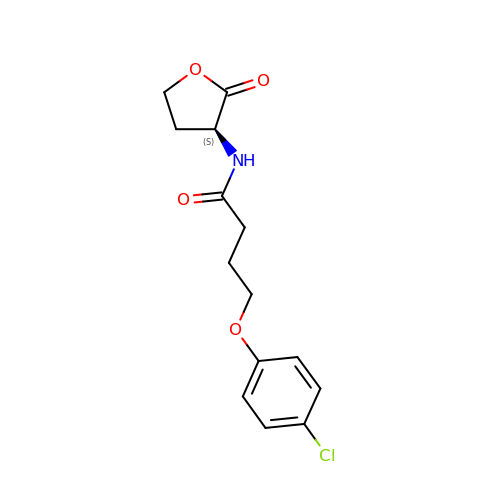4-(4-chlorophenoxy)-N-[(3S)-2-oxotetrahydrofuran-3-yl]butanamide | C14 H16 Cl N O4 | BKVYYPQMGSVOHB-LBPRGKRZSA-N2-ETHOXYETHANOL | C4 H10 O2 | 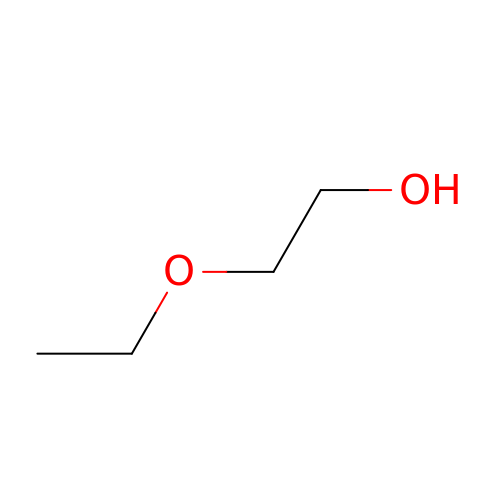ZNQVEEAIQZEUHB-UHFFFAOYSA-N>[2x]MNVELFKKFSEKVEEIIEAGRILHSRGWVPATSGNISAKVSEEYIAITASGKHKGKLTPEDILLIDYEGRPVGGGKPSAETLLHTTVYKLFPEVNA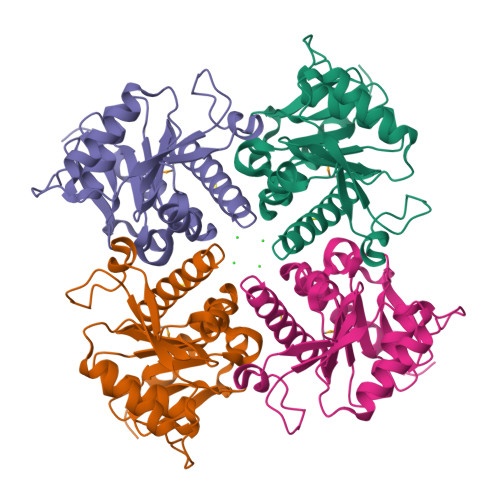VVHTHSPNATVISIVEKKDFVELEDYELLKAFPDIHTHEVKIKIPIFPNEQNIPLLAKEVENYFKTSEDKYGFLIRGHGLYTWGRSMEEALIHTEALEFIFECELKLLSFHS>[4x]SANEDMPVERILEAELAVEPKTETYVEANMGLNPSSPNDPVTNICQAADKQLFTLVEWAKRIPHFSELPLDDQVILLRAGWNELLIASFSHRSIAVKDG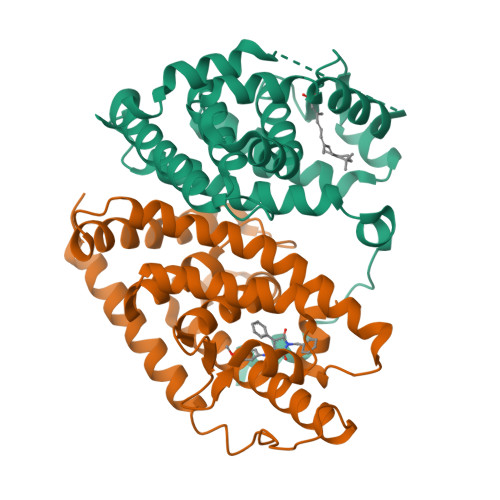ILLATGLHVHRNSAHSAGVGAIFDRVLTELVSKMRDMQMDKTELGCLRAIVLFNPDSKGLSNPAEVEALREKVYASLEAYCKHKYPEQPGRFAKLLLRLPALRSIGLKCLEHLFFFKLIGDTPIDTFLMEMLEAPHQMT;>VQLSPEQLGMIEKLVAAQQQCNRRSFSDRLRVTPWPIAPDPQSREARQQRFAHFTELAIVSVQEIVDFAKQLPGFLQLSREDQIALLKTSAIEVMLLETSRRYNPGSESITFLKDFSYNREDFAKAGLQVEFINPIFEFSRAMNELQLNDAEFALLIAISIFSADRPNVQDQLQVERLQHTYVEALHAYVSINHPHDPLMFPRMLMKLVSLRTLSSVHSEQVFALRLQDKKLPPLLSEIWDVHE[4x]> KTPPVYPVTVPFLGHIVQFGKNPLEFMQRCKRDLKSGVFTISIGGQRVTIVGDPHEHSRFFSPRNEILSPREVYTIMTPVFGEGVAYAAPYPRMREQLNFLAEELTIAKFQNFVPAIQHEVRKFMAENWKEDEGVINLLEDCGAMIINTACQCLFGEDLRKRLNARHFAQLLSKMESSLIPAAVFMPWLLRLPLPQSARCREARAELQKILGEIIVAREKEEASKDNNTSDLLGGLLKAVYRDGTRMSLHEVCGMIVAAMFAGQHTSTITTSWSMLHLMHPKN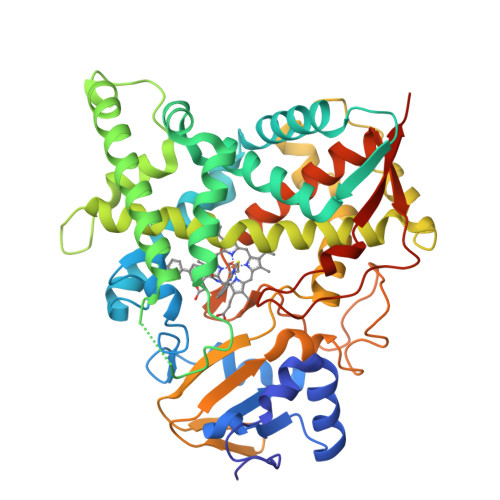KKWLDKLHKEIDEFPAQLNYDNVMDEMPFAERCVRESIRRDPPLLMVMRMVKAEVKVGSYVVPKGDIIACSPLLSHHDEEAFPNPRLWDPERDEKVDGAFIGFGAGVHKCIGQKFALLQVKTILATAFREYDFQLLRDEVPDPDYHTMVVGPTLNQCLVKYTRKKKLPSHHHHHH> MNRIAEAFEELKKKGEKALIPFITAGDPDLETTLELVRALVEAGADIIELGIPFSDPLADGP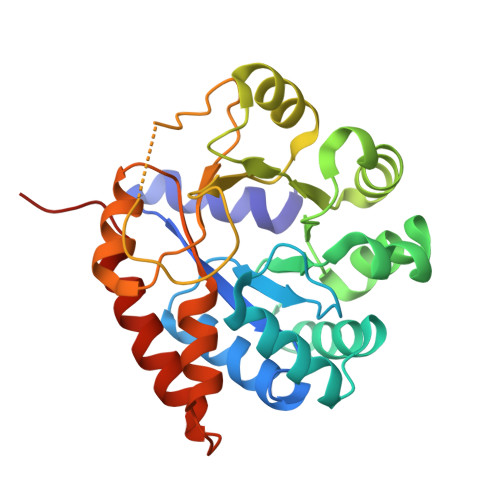TIQRASQRALASGTTLDKVFEMVRELREKNTDVPIVFLTYYNPIFRYGIERFVKECAEAGVDGLIVPDLPPEEAADLAAAAEKYGVDLIFLVAPTSTDERIKMIAKHASGFVYCVSVTGVTGARSEIAADLAELVSRIRKHTDLPIAVGFGISTPEQAAEVAQVADGVIVGSAIVKRIEENQDEEDIVEEVREFVRELREAVKLEHHHHHH>[2x]MLEVVTAGEPLVALVPQEPGHLRGKRLLEVYVGGAEVNVAVALARLGVKVGFVGRVGEDELGAMVEERLRAEGVDLTHFRRAPGFTGLYLREYLPLGQGRVFYYRKGSAGSALAPGAF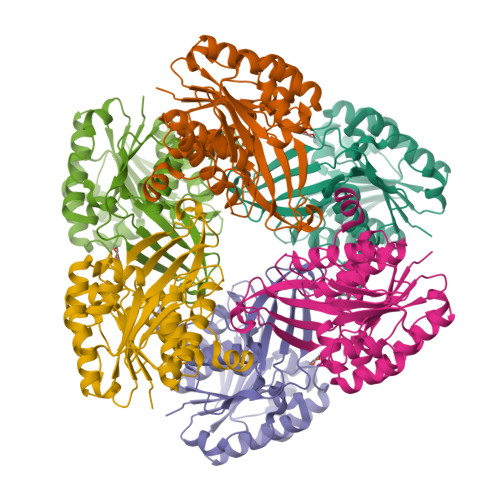DPDYLEGVRFLHLSGITPALSPEARAFSLWAMEEAKRRGVRVSLDVNYRQTLWSPEEARGFLERALPGVDLLFLSEEEAELLFGRVEEALRALSAPEVVLKRGAKGAWAFVDGRRVEGSAFAVEAVDPVGAGDAFAAGYLAGAVWGLPVEERLRLANLLGASVAASRGDHEGAPYREDLEVLLKATQTFMR> MSESEAKSRSATPPSKAKQATPTTTAAANGEKKLTNKELKELKKQEKAAKRAAMKQANGISIEQQQQQAQMKKEKKQLQREQQQKREQKQKNANKKKQNERNVKKSTLFGHLETTEERRATILALTSAVSSPKTSRITAAGLMVPVVASALSGSNVLTASSLMPVGPNASSTVSASAPASTTTTLPASSAALSAGTSSASTNTPTAIQQEIASSNASDVAKTLASISLEAGEFNVIPGISSVIPTVLEQSFDNSSLISSVKELLLNKDLIHPSILLLTSHLAHYKIVGSIPRCIAMLEVFQIVIKDYQTPKGTTLSRNLTSYLSHQIDLLKKARPLSVTMGNAIRWLKQEISLIDPSTPDKAAKKDLCEKIGQFAKEKIELADQLIIDNASTQIEESTTIVTYGSS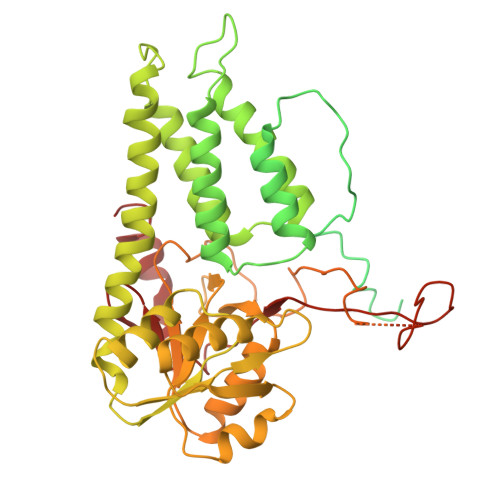KVLTELLLHNAISLKKNIKVIVVDSRPLFEGRKMAETLRNAGVNVMYALITSLDTIFNMDVDYVFLGAHSILSNGFLYSRAGTAMLAMSAKRRNIPVLVCCESLKFSQRVQLDSVTFNELADPNDLVNIDYENPVERRGNKGALLNQFIKERKFEKKKLAMENKPKGNKIGGKKGSEGESKDASNEEDSNSKNILDGWQELPSLNIVNILYDLTPPEYIKKVITEFGALPPSSVPVILREYKGSA>MQIGFIGVGLMGGPLARNLIRAGKDVTVYDLSPEAVKKTLAAGNTGKAAASLADLADKDIVFTSLPLPTHVLGVVLGNDGLLEKLKPGATHIELSTIDPQTSVKLEAAARAKGCHFLQCTLGKTPAHAEKAEEPLFIGGDKAIFDELAALWPIIGSPAYYMGTVEASCAVKLISNMVGMTN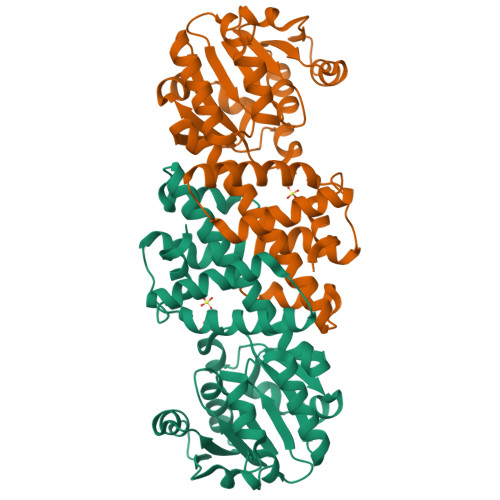LAVLAEGIRIGEKAGIKRSQLLTLLQDTGARSFQMDVRGPWIANDDFANRFGLDLALKDVRLGCEMAEAWGMKIPAMMAALGIFKKASATGLGSEDCNAIYKVTE[3x]>MNHKVHMMSQPKPILYYDERSPPVRSCLMLIKLLDIDVELRFVNLFKGEQFQKDFLALNPQHSVPTLVHGDLVLTDSHAILIHLAEKFDEGGSLWPQEHAERMKVLNLLLFECSFLFRRASDFMSAIVRQGFANVDVAHHERKLTEAYIIMERYLENSDFMAGPQLTLADLSIVTTLSTVNLMFPLSQFPR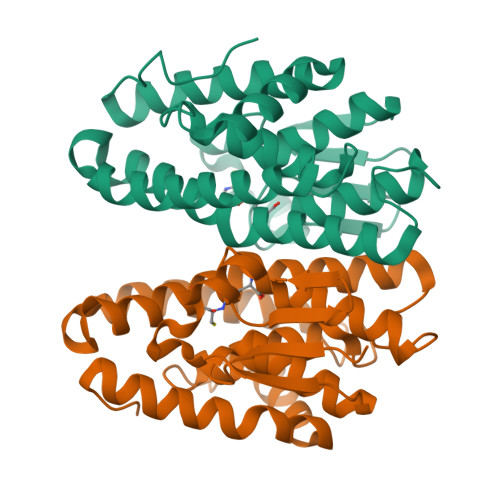LRRWFTAMQQLDAYEANCSGLEKLRQTMESVGSFQFPSSSAVVTEKVE[2x]>[2x]TELTKCKVSHAIKDI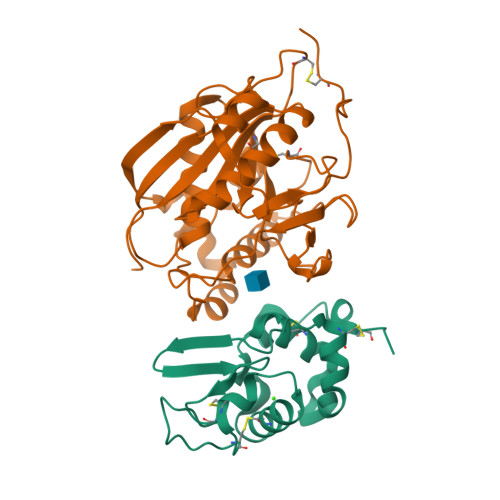DGYQGISLLEWACVLFHTSGYDTQAVVNDNGSTEYGLFQISDRFWCKSSEFPESENICGISCDKLLDDELDDDIACAKKILAIKGIDYWKAYKPMCSEKLEQWRCEKP;>ASMTGGQQMGRGSSLTACPEESPLLVGPMLIEFNIPVDLKLVEQQNPKVKLGGRYTPMDCISPHKVAIIIPFRNRQEHLKYWLYYLHPILQRQQLDYGIYVINQAGESMFNRAKLLNVGFKEALKDYDYNCFVFSDVDLIPMNDHNTYRCFSQPRHISVAMDKFGFSLPYVQYFGGVSALSKQQFLSINGFPNNYWGWGGEDDDIYNRLAFRGMSVSRPNAVIGKCRMIRHSRDKKNEPNPQRFDRIAHTKETMLSDGLNSLTYMVLEVQRYPLYTKITVDIGTPS[2x]> NLVQFGVMIEKMTGKSALQYGDYGCYCGIGGSHWPVDQTDWCCHAHDCCYGRLEKLGCEPKLEKYLFSVSERGIFCAGRTTCQRLTCECDKRAALCFRRNLGTYNRKYAHYPNKLCTGPTPPC

The mammalian family of secreted phospholipase A2 (sPLA2), which are Ca2+ dependent, low-molecular weight and disulfide-rich enzymes, plays key roles in many physiological functions and pathological processes by catalyzing the hydrolysis of phospholipids at the sn-2 position. GIIE, the closest homolog to GIIA, is regarded as a “hair follicular”, “inflammatory” and “metabolic” sPLA2. The structure of hGIIE consists of a typical set of three major helices (α1, α3 and α4), two β-strands (β1 and β2), and three short helices (α2, α5 and α6) around the second calcium binding site. Similar to hGIIA, hGIIE has seven disulfide bonds.

To study the role of Asn21 in the enzymatic activity of hGIIE, we designed hGIIE variants, including N21G (mimicking hGIIA and hGV), N21M (mimicking hGX) and N21W (mimicking hGIID). For hGIIA, Gly21 can neither form the hydrogen bond nor clash with these compounds. For hGIIE, these compounds present 2–24 fold decreased inhibition effect against mutant N21G compared to the WT hGIIE. Our results on the co-crystal structure of hGIIE N21G mutant with compound 24 also confirm that the inhibitor binds much weaker to the mutant protein than the WT protein. Compound 24 in N21G structure has poor Fo-Fc map compared to the WT structure, and the occupancy of compound 24 in N21G structure is refined to only 68%. Therefore, Asn21 in hGIIE is one critical residue contributed to the best effect of these indole analogues against hGIIE.> IQVTQPSVVLASSHGVASFPCEYSPSHNTDEVRVTVLRQTNDQMTEVCATTFTEK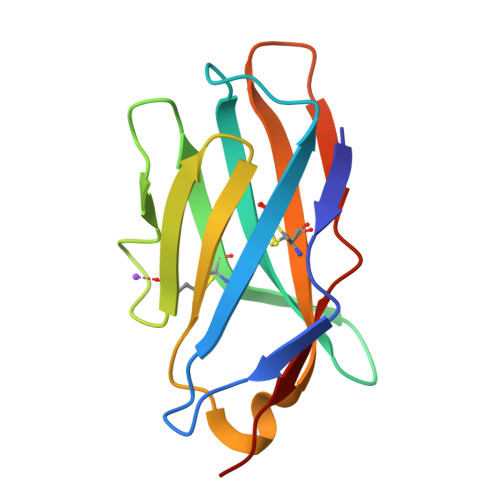NTVGFLDYPFCSGTFNESRVNLTIQGLRAVDTGLYLCKVELMYPPPYFVGMGNGTQIYVIDP>[2x]GSMALFSAQSPYINPIIPFTGPIQGGLQEGLQVTLQGTTKSFAQRFVVNFQNSFNGNDIAFHFNPRFEEGGYVVCNTKQNGQWGPEERKMQMPFQKGMPFELCFLVQRSEFKVMVNKKF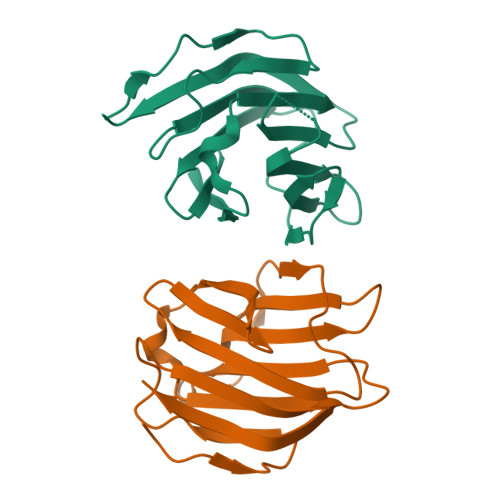FVQYQHRVPYHLVDTIAVSGCLKLSFITFQTQNFRPAHQA>[4x]MDMTQQEIFDKQRRL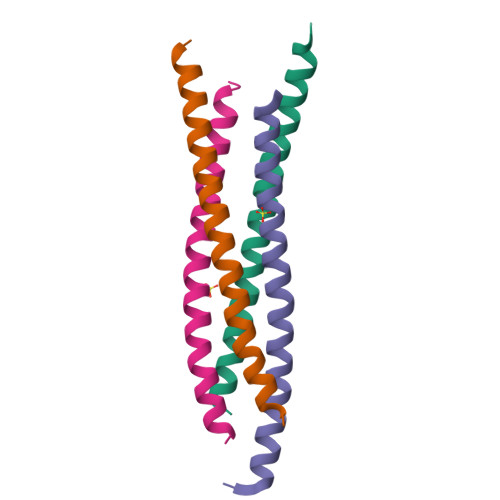QELSEKVRTCHQEASALRKAAQEKEAEMLQVLEDIQTI3N methyl nemycin B | C24 H48 N6 O13 | 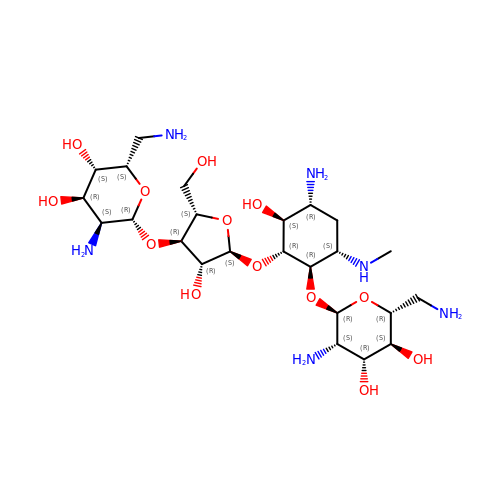FCJYTWXMZQXWFB-HGRVKHENSA-N>[2x]RSLVSVHNEWDPLEEVIVGTAVGARVPTADRSVFAVE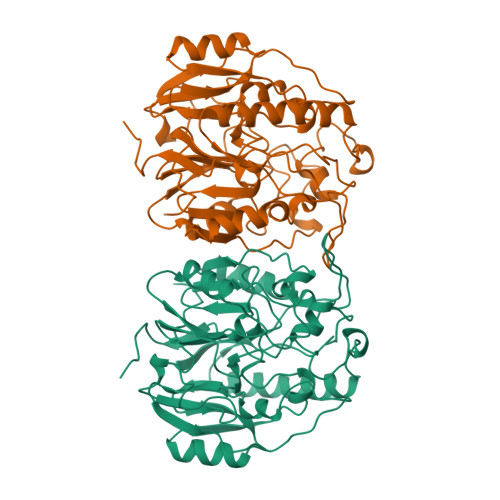YAGDYESQEQIPSGAYPDRVLKETEEELHVLAAELTKLGVTVRRPGPRDHSALIKTPDWETDGFHDYCPRDGLLSVGQTIIETPMALRSRFLESLAYKDLLLEYFASGSRWLSAPKPRLTDDSYAPQAPAGERLTDEEPVFDAANVLRFGTDLLYLVSDSGNELGAKWLQSAVGDTYTVHPCRKLYASTHVDSTIVPLRPGLVLTNPSRVNDENMPDFLRSWENITCPELVDIGFTGDKPHCSVWIGMNLLVVRPDLAVVDRRQTALIRLLEKHGMNVLPLQLTHSRTLGGGFHCATLDVRRTGALETYQF>[3x]MHHHHHHHHHHHHMMESGAPICHTCGEQVGHDANGDLFVACHECNYHICKSCFEYEIKEGRKVCLRCGSPYDENLLDDVEKKGSGNQSTMASHLNNSQDVGIHARHISSVSTVDSEMNDEYGNPIWKNRVESWKDKRNKKKKSNTKPETEPAQVPPEQQMENKPSAEASEPLSIVYPIPRNKLTPYRAVIIMRLIILGLFFHYRITNPVDSAFGLWLTSVICEIWFAFSWVLDQF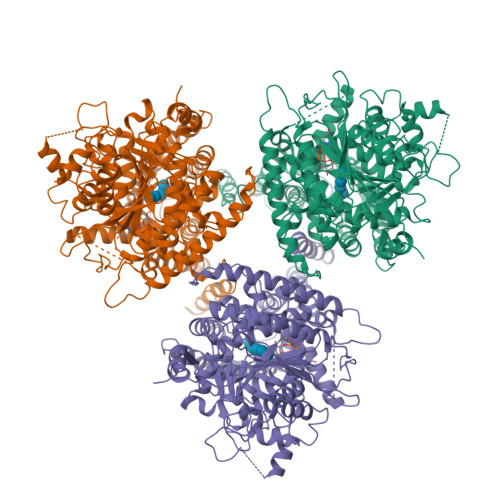PKWKPVNRETFIERLSARYEREGEPSQLAAVDFFVSTVDPLKEPPLITANTVLSILAVDYPVDKVSCYVSDDGAAMLTFESLVETAEFARKWVPFCKKFSIEPRAPEFYFSQKIDYLKDKVQPSFVKERRAMKRDYEEYKVRVNALVAKAQKTPDEGWTMQDGTPWPGNNTRDHPGMIQVFLGNTGARDIEGNELPRLVYVSREKRPGYQHHKKAGAENALVRVSAVLTNAPYILNLDCDHYVNNSKAVREAMCILMDPQVGRDVCYVQFPQRFDGIDRSDRYANRNIVFFDVNMKGLDGIQGPMYVGTGCVFNRQALYGYGPPSMPRLRKGKESSSCFSCCCPTKKKPAQDPAEVYRDAKREDLNAAIFNLTEIDNYDDYERSMLISQLSFEKTFGLSPVFIESTLMENGGVPESANSSTLIKEAIHVIGCGFEEKTEWGKEIGWIYGSVTEDILSGFKMHCRGWRSIYCMPVRPAFKGSAPINLSDRLHQVLRWALGSVEIFFSRHCPFWYGYGGGRLKWLQRLAYINTIVYPFTSLPLIAYCTIPAVCLLTGKFIIPTLSNLASMLFLGLFISIIVTAVLELRWSGVSIEDLWRNEQFWVIGGVSAHLFAVFQGFLKMLAGIDTNFTVTAKAADDTEFGELYMVKWTTLLIPPTTLLIINIVGVVAGFSDALNKGYEAWGPLFGKVFFAFWVILHLYPFLKGLMGRQNRTPTIVVLWSVLLTSVFSLVWVKINPFVNKVDNTLAGETCISIDC The multiple inositol polyphosphate phosphatases (MINPPs) constitute a distinct evolutionary group within clade 2 of the histidine phosphatase superfamily. To gain a wider understanding of the implications of these insertions on the properties of these enzymes, we carried out a crystal structure and mutagenic analysis of a representative member, BlMINPP, a moderately thermophilic, membrane-anchored extracellular enzyme. In keeping with previously reported crystal structures of HP2P family members, the structure of BlMINPP consists of two domains, an α/β-domain and an α-domain. The catalytic center of BlMINPP consists of the nucleophilic histidine (His-45), three arginine residues (Arg-44, Arg-48, and Arg-142), which coordinate the scissile phosphate during catalysis, and the amino acid triplet HAE (residues 339-401) where the glutamic acid residue acts as the presumed proton donor during catalysis.

To this end, crystals of the apoenzyme and of an inactive mutant in which the presumed catalytic proton donor Glu-401 was replaced by a glutamine (E401Q) were prepared, the latter in an attempt to trap the catalytic phosphohistidine intermediate. The structures of the apoenzyme and product complex were solved at 1.65 and 1.71 Å resolution, respectively, whereas a data set collected at 2.40 Å resolution from a crystal of the inactive E401Q mutant yielded a structure of the His-45 phosphohistidine derivative. In the phosphohistidine intermediate, Arg-48 and Arg-142 adopt open-state conformations, neither making contact with the His-45 phospho-group. In fact, this group does not make contact with hinge residues and makes direct contact only with the main chain amide of A400 (A400 forms part of the HAE proton donor motif). It also forms a weaker interaction with Arg-44. The loss of the majority of the interactions observed with the scissile phosphate in the substrate complex are consistent with the relaxation of the phosphohistidine intermediate enzyme to the fully open state. Unexpectedly, the phosphohistidine intermediate state resembles the open conformation, whereas the product-bound form of the enzyme exhibits a lid rotation of 10° (degree of closure 68.6%) back to a half-closed conformation. Taken together, these snapshots suggest a mechanism whereby the enzyme undergoes a complex structural catalytic cycle during which the lid closes on binding of substrate, then opens fully to expel the first stage product (a lower phosphorylated inositol). Restoration of the open state conformation in the phosphohistidine intermediate allows product egress, before return to a half-closed state to allow breakdown of the intermediate and generation of the second stage product, orthophosphate.

>[2x]GSHMASMEADGRYYSSKQPYVAPNDATASSYSKAPKGYGPIYTESMARHGSRGLSSYKYDALLMRMAETAARDGGFKSEAIKAEFVKNLSGITAANVENGYGMLTGQGAQQHYGIGERAYQRNRSLFDQAAADGGTIAYQSSGEARATESGENFEKGFNEASGGRLIGNVSAPTNPADSGNGKDFQKNPDTLYFHKVQNPDGTSKVPGTKAYDIANNYQNFVANDATIAGAEKTIGDNVDVKRASHDLLSQIFTEEFLAKLENGEYKWYNTTDGTKKGGKNCAPGADASKDPDACGEVSKKIKSEYDAAMDLYNLYIIAADMHNENTGDHTFAFDQYFQGAYADDARMFAWALDAEDFYEKGPSYAGQNETYSIAQPLLDDFLNTIDARVNGGSTVATFRFAHAQTMMPFAALLGLPGSTQQAPASTTDVYTYGNNEWRGESVTPMAANVQWDVYARKGEDPATGQRYTPIVRMLYNENEVPFRSECTPVADGSTWYKLTELKSCLAADHKTLGQDARI>[3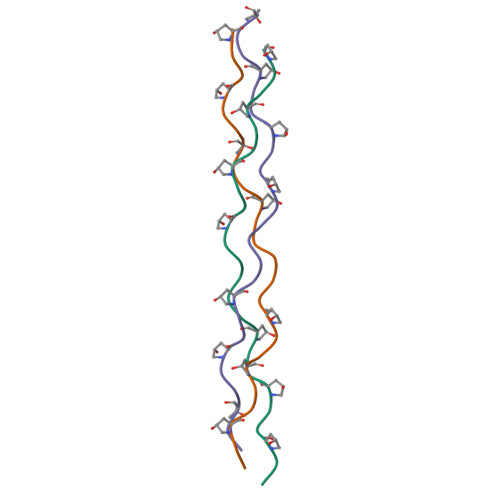x]XGPPGPPGPPGKLGPPGPPGPPGPPX>[2x]MIIDYFDNESINEDIKNYIQRRIKAYGDLRYSYLVMNKKTPLHPTIISNY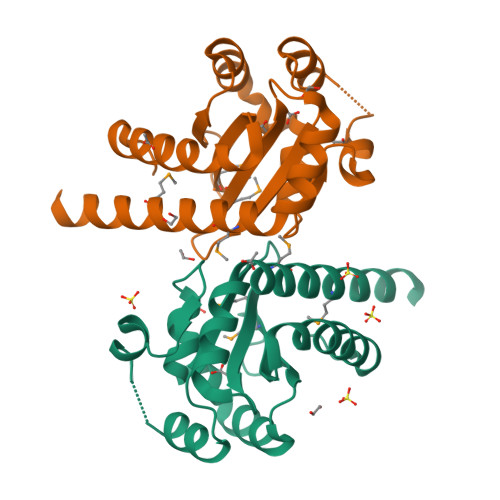PLDWVKKYKKNSYHLIDPVILTAKDKVAPFAWDDNSVINKKSTDSAVFKLAREYNIVNGYTFVLHDNSNNMATLNISNGSDDSISFDESIEINKEKIQMLLILTHEKMLGLYQSNSDKNENRNPKIERD>[2x]PITGLVYDQRMMLHHNMWDSHHPELPQRIS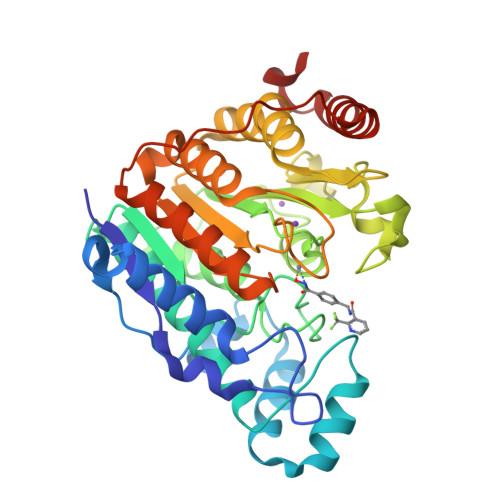RIFSRHEELRLLSRCHRIPARLATEEELALCHSSKHISIIKSSEHMKPRDLNRLGDEYNSIFISNESYTCALLAAGSCFNSAQAILTGQVRNAVAIVRPPGHHAEKDTACGFCFFNTAALTARYAQSITRESLRVLIVDWDVHHGNGTQHIFEEDDSVLYISLHRYEDGAFFPNSEDANYDKVGLGKGRGYNVNIPWNGGKMGDPEYMAAFHHLVMPIAREFAPELVLVSAGFDAARGDPLGGFQVTPEGYAHLTHQLMSLAAGRVLIILEGGYNLTSISESMSMCTSMLLGDSPPSLDHLTPLKTSATVSINNVLRAHAPFWSSLR> SNAEKRKYQIRYATVNDIPNLLKCATFNQPVNEPFFQVLLKQTPTAHLLLEYQGELVAAIFTETKNSNEVLGIREFLVRTSVENWQVLAKDLLEFVEQWGVVKPGIKEIEGLLKYHEAISNFQKSKWYQSSVLNKKLIEKITLHELATLELCNLMAPEYELEAFAAR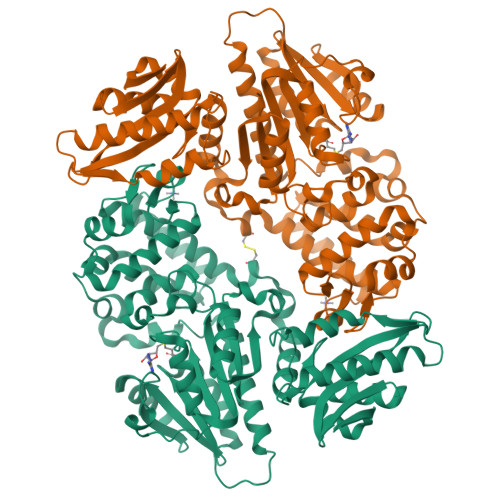WLLRVFQDMGVFLREGESYQESELVSQLNISPRYQRLLGALLQILHKRGILKIEKDRVFTLARCKTFALENISSEVSAFYDYFSEKYPAHLSWLTVVKRCLEKYPLILRGEVDVNEVVFTDGDMELFAGLFLGHRVADYFNELLADGVCWEVEQRLLEEKRAQPIRILEIGAGTGGVTGILLEKLASHAEQIEFWFTDISSVFTRYGESKFKQFPWVKYQTFDIEKSLDAQGIKSESFDVVIANNVLHNTKLIHQTLNNSNSLLNTGGLLALLEFTQPIDILLYFGGLLQGFWLFEDPEYRLEVGCLLSIPLWQKVLSDCGFDEIIPLGLPCEMHALSKARESVIFARKHQVQEKT>[3x]MIKIKLTHPDCMPKIGSEDAAGMDLRAFFGTNPAADLRAIAPGKSLMIDTGVAVEIPRGWFGLVVPRSSLGKRHLMIANTAGVIDSDYRGTIKMNLYNYGSEMQTLENFERLCQLVVLPHYSTHNFKIVDELEETIRGEGGFGSSGSK

Deoxyuridine triphosphate nucleotidohydrolases (dUTPases, or Duts) are produced by most living organisms as part of their pyrimidine biosynthesis networks. Their role is to eliminate excess dUTP, which can be mistakenly incorporated into DNA by DNA polymerases, since most of them cannot distinguish between dUTP and dTTP. In addition, dUTPases provide the dTTP precursor, dUMP. In this study, we demonstrate for the first time that the homotrimeric dUTPase of bacteriophage T5 performs an additional, non-enzymatic function in the virus’s life cycle.

We determined the crystal structure of bacteriophage T5 dUTPase with a resolution of 2.0 Å, and we discovered a distinct short loop consisting of six amino acid residues, representing a unique structural feature specific to the T5-like phages dUTPases. The comparative analysis of dUTPase sequences from bacteriophage T5 and the host organism E. coli revealed a low identity of only 34%. Despite the low identity, the overall tertiary and quaternary dUTPase structures of the phage and host were found to be very similar, with a root-mean-square deviation (RMSD) of 1.3 Å when aligning the Cα atoms of the monomers. Although there is limited sequence similarity between the T5 phage dUTPase (T5Dut) and the E. coli dUTPase, the comparison of their spatial structures revealed a high degree of similarity, except for the presence of a specific loop in the T5 and T5-like phages that is absent in the bacterial protein. The structure shows the typical trimeric dUTPase antiparallel β-pleated fold of the subunits. Three subunits are attached to each other in the same manner as observed in other trimeric dUTPases, forming three active sites per enzyme molecule in the region of monomer interaction. A comparison of the amino acid sequence and structure of the T5Dut phage with other characterized enzymes allowed us to identify two conserved amino acid residues (Ser68 and Asp85) within the active site that are directly involved in the enzymatic reaction in T5Dut. We have identified a structural element within T5Dut, a small-loop 30-GTNPAA-35 that is only six amino acids long, which is responsible for the implementation of a novel function.>[2x]MIIYRDLISHDEMFSDIYKIREIADGLCLEVEGKMVSRTEGNIDDSLIGGNASAEGPEGEGTESTVITGVDIVMNHHLQETSFTKEAYKKYIKD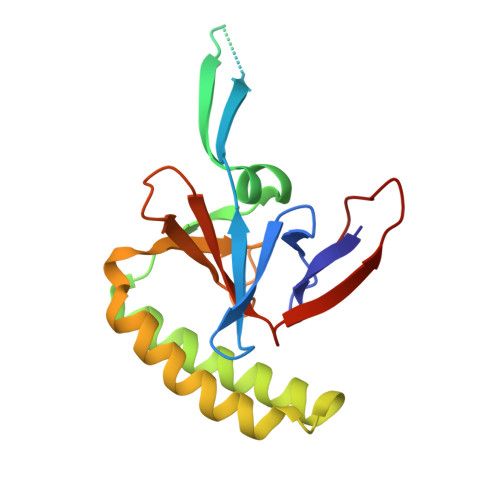YMKSIKGKLEEQRPERVKPFMTGAAEQIKHILANFKNYQFFIGENMNPDGMVALLDYREDGVTPYMIFFKDGLEMEKCLEHHHHHH>[4x]MASVQLQNVTKAWGEVVVSKDINLDIHEGEFVVFVGPSGCGKSTLLRMIAGLETITSGDLFIGEKRMNDTPPAERGVGMVFQSYALYPHLSVAENMSFGLKLAGAKKEVINQRVNQVAEVLQLAHLLDRKPKALSGGQRQRVAIGRTLVAEPSVFLLDEPLSNLDAALRVQMRIEISRLHKRLGRTMIYVTHDQVEAMTLAD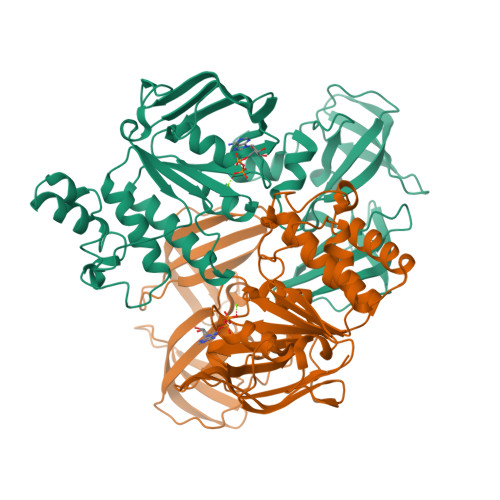KIVVLDAGRVAQVGKPLELYHYPADRFVAGFIGSPKMNFLPVKVTATAIDQVQVELPMPNRQQVWLPVESRDVQVGANMSLGIRPEHLLPSDIADVILEGEVQVVEQLGNETQIHIQIPSIRQNLVYRQNDVVLVEEGATFAIGLPPERCHLFREDGTACRRLHKEPGVASASHHHHHH> CVICDPSVVLALKSLEKDYLPGHLDAKHHKAMMERVENAVKDFQELSLNEDAYMGVVDEATLQKGSWSLLKDLKRITDSDVKGDLFVKELFWMLHLQKETFATYVARFQKEAYCPNKCGVMLQTLIWCKNCKKEVHACRKSYDCGER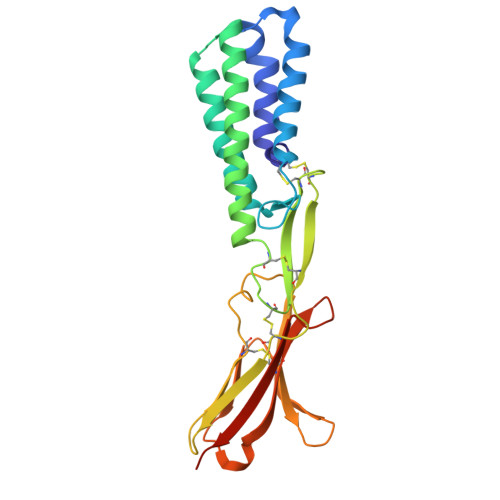NVEVPQMEDMILDCELNWHQASEGLTDYSFYRVWGNNTETLVSKGKEATLTKPMVGPEDAGSYRCELGSVNSSPATIINFHVTVLPGRAVPR Human ATP:cob(I)alamin adenosyltransferase (ATR) is a mitochondrial enzyme that catalyzes an adenosyl transfer to cob(I)alamin, synthesizing 5′-deoxyadenosylcobalamin (AdoCbl) or coenzyme B12. ATR is also a chaperone that escorts AdoCbl, transferring it to methylmalonyl-CoA mutase, which is important in propionate metabolism. Mutations in ATR lead to methylmalonic aciduria type B, an inborn error of B12 metabolism. Human ATR is a homotrimer with active sites that are located at the subunit interfaces.

To gain structural insights into how the mutations impact AdoCbl binding, R190C and E193K ATR were cocrystallized with AdoCbl and PPPi, and the structures were solved by molecular replacement. Electron density that could be modeled as AdoCbl but not PPPi was present in the 1.8 Å structure of R190C and 2.2 Å structure of E193K ATR·AdoCbl. Both had four identical chains per asymmetric unit with an occupancy of one AdoCbl per monomer. Structural overlays revealed Cα RMSD values of 1.6 Å and 1 Å for WT ATR·ATP versus R190C·AdoCbl and E193K·AdoCbl, respectively, indicating that the mutations do not induce major conformational changes in the overall structure. More of the N-terminus was disordered, and both structures were resolved after residue-79, as previously seen with WT ATR·AdoCbl. AdoCbl was bound in the base-off conformation with Phe-170 positioned at a distance of 3.6 Å from the cobalt atom. An overlay of the WT and R190C ATR structures revealed subtle differences in the position of the ribose ring. In WT ATR, the side chain of Arg-190 interacts via salt bridges to the ribose oxygen and the C6 amino group of the deoxyadenosine moiety. The mutation replaces the salt bridges by a hydrogen-bonding network between Cys-190 and the ribose oxygen that is mediated via two water molecules. Like WT ATR, all three mutants bound AdoCbl in the base-off state but with affinities that were 40- (R190C), 50- (R190H) and 120- (E193K) fold weaker respectively.

>MPKIYTKTGDKGFSSTFTGERRPKDDQVFEAVGTTDELSSAIGFALELVTEKGHTFAEELQKIQCTLQDVGSALATPCSSAREAHLKYTTFKAGPILELEQWIDKYTSQLPPLTAFILPSGGKISSALHFCRAVCCRAERRVVPLVQMGETDANVAKFLNRLSDYLFTLARYAAMKEGNQEKIYMKNDPSAESEGL[4x]> TGREILEKLERREFTREVLKEALSINDRGFNEALFKLADEIRRKYVGDEVHIRAIIEFSNVCRKNCLYCGLRRDNKNLKRYRMTPEEIVERARLAVQFGAKTIVLQSGEDPYYMPDVISDIVKEIKKMG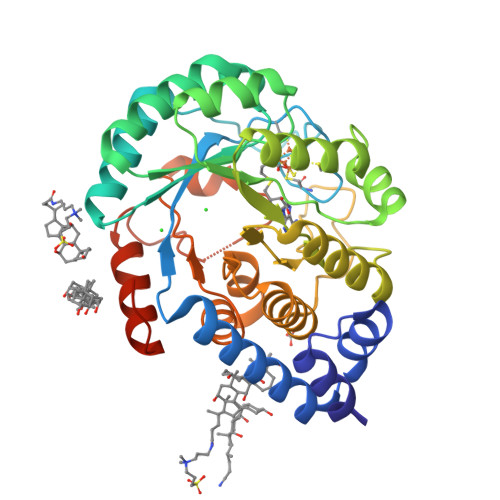VAVTLSLGEWPREYYEKWKEAGADRYLLRHETANPVLHRKLRPDTSFENRLNCLLTLKELGYETGAGSMVGLPGQTIDDLVDDLLFLKEHDFDMVGIGPFIPHPDTPLANEKKGDFTLTLKMVALTRILLPDSNIPATTAMGTIVPGGREITLRCGANVIMPNWTPSPYRQLYQLYPGKICVFEKDTACIPCVMKMIELLGRKPGRDWGGRKRVFETV>MPFEVVFDGAKEFADLIATASNLIDEAAFKFTEEGISMRAMDPSRVVLIDLNLPESIFSKYEVEEPETIGINMDQFKKILKRGKAKDTLILRKGDENFLEITFEGTAKRTFRLPLIDVEELELELPELPFTAKVVLLGEVLKEGIKDASLVSDAIKFIAKENEFTMKAEGETNEVEIRLTLEDEGLLDLEVEEETKSAYGIRYLSDMVKGIGKADEVILRFGNEMPLQMEYMIRDEGRLTFLLAPRVEEHHHHHH[2x];>MDRKLDEFIGDATPKKVSKEKPVRRKKRLKPTSLDSFLPEEHINYFRDL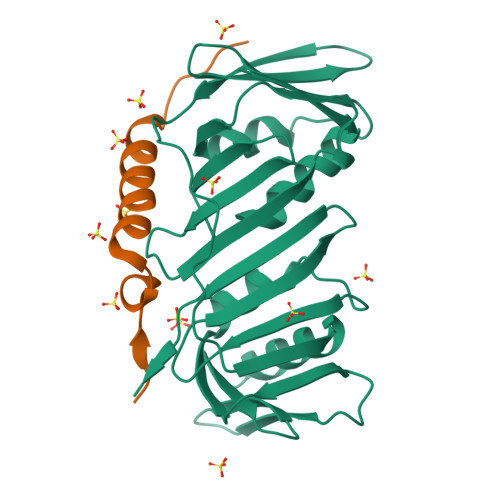RIGSKKIRNAKIEEL[2x]FGAR-AT encoded by the purL gene is a multidomain bi-functional enzyme that catalyzes the fourth step of the purine biosynthesis pathway. The FGAR-AT protein from Salmonella typhimurium (StPurL) has 1295 amino acid residues and is a single chain protein with three major domains. The C-terminal glutaminase domain produces an ammonia molecule that is consumed at the coupled active site present in the formylglycinamidine ribonucleotide (FGAM) synthetase domain where nitrogen is incorporated into an FGAR molecule converting it into FGAM. While the FGAM synthetase domain and glutaminase domain carry out the two enzymatic reactions within this bi-functional enzyme, the function of the N-terminal domain is not clearly understood.

However, F209W mutation that was expected to block the cavity at the expense of some clashes with the adjacent Leu182 and Glu186 residues was made. Surprisingly, the F209W mutation was very successful and had expression and purification profile at par with the wild-type. The crystal structure of this protein was solved by molecular replacement at 1.5 Å resolution. The mFo-DFc map depicted clear density for the tryptophan residue that had adjusted into the structure by adopting a similar conformation to that of the phenylalanine residue it replaced. Per residue rmsd of the region around the Xe3 binding cavity was calculated between the F209W mutant and the StPurL-Xenon complex and it was found that mutagenesis at position 209 resulted in a local readjustment of the structure. To accommodate the larger tryptophan residue, side chains of amino acids in close proximity of the original phenylalanine residue like Glu186 and Leu182 residing on helix α7 readjusted adopting alternate rotamers. The surface exposed lysine residue, Lys608 residing on a loop spanning residues 601–613 which, lines the Xe cavity has the highest overall residue rmsd value of 1.7 Å. This loop showed maximum perturbation of the backbone in the mutant structure and is a part of the long linker region (601–631) that connects the B1 and the B2 sub-domains. Other residues in this region with average rmsd over all atoms greater than 1 Å were Glu184, Glu186 and Lys196. This result demonstrates that local perturbations in structure can translate into movement of residues in the outer shell of the cavity by propagating adjustments in surface residues and that cavity 3 exhibits structural plasticity. Out of the three internal hydrophobic spaces marked by xenon atoms, the region around the third xenon site was found to be most malleable and tolerant to mutagenesis. This site was more surface exposed and although mutation of F209W resulted in perturbation of the local environment, the changes were tolerated as is evident from the crystal structure.

> GDGLVPRGSHMMEILRGSPALSAFRINKLLARFQAANLQVHNIYAEYVHFADLNAPLNDSEQAQLTRLLQYGPALSSHTPAGKLLLVTPRPGTISPWSSKATDIAHNCGLQQVDRLERGVAYYIEASTLTAEQWRQVAAELHDRMMETVFSSLTDAEKLFIHHQPAPVSSVDLLGEGRQALIDANLRLGLALAEDEIDYLQEAFTKLGRNPNDIELYMWAQANSEHCRHKIFNADWIIDGKPQPKSLFKMIKNTFETTPDYVLSAYKDNAAVMEGSAVGRYFADHNTGRYDFHQEPAHILMKVETHNHPTAISPWPGAATGSGGEIRDEGATGRGAKPKAGLVGFSVSNLRIPGFEQPWEEDFGKPERIVTALDIMTEGPLGGAAFNNEFGRPALTGYFRTYEEKVNSHNGEELRGYHKPIMLAGGIGNIRADHVQKGEIVVGAKLIVLGGPAMNIGLGGGAASSMASGQSDADLDFASVQRDNPEMERRCQEVIDRCWQLGDANPILFIHDVGAGGLSNAMPELVSDGGRGGKFELRDILSDEPGMSPLEIWCNESQERYVLAVAADQLPLFDELCKRERAPYAVIGDATEEQHLSLHDNHFDNQPIDLPLDVLLGKTPKMTRDVQTLKAKGDALNRADITIADAVKRVLHLPTVAEKTFLVTIGDRTVTGMVARDQMVGPWQVPVADCAVTTASLDSYYGEAMSIGERAPVALLDFAASARLAVGEALTNIAATQIGDIKRIKLSANWMAAAGHPGEDAGLYDAVKAVGEELCPQLGLTIPVGKDSMSMKTRWQEGNEQREMTSPLSLVISAFARVEDVRHTLTPQLSTEDNALLLIDLGKGHNALGATALAQVYRQLGDKPADVRDVAQLKGFYDAMQALVAARKLLAWHDRSDGGLLVTLAEMAFAGHCGVQVDIAALGDDHLAALFNEELGGVIQVRAEDRDAVEALLAQYGLADCVHYLGQALAGDRFVITANDQTVFSESRTTLRVWWAETTWQMQRLRDNPQCADQEHEAKANDTDPGLNVKLSFDINEDIAAPYIATGARPKVAVLREQGVNSHVEMAAAFHRAGFDAIDVHMSDLLGGRIGLGNFHALVACGGFSYGDVLGAGEGWAKSILFNHRVRDEFETFFHRPQTLALGVCNGCQMMSNLRELIPGSELWPRFVRNHSDRFEARFSLVEVTQSPSLLLQGMVGSQMPIAVSHGEGRVEVRDDAHLAALESKGLVALRYVDNFGKVTETYPANPNGSPNGITAVTTENGRVTIMMPHPERVFRTVANSWHPENWGEDSPWMRIFRNARKQLG>[2x]RPSGRKSSKMQAFRIWDVNQKTFYLRNNQLVAGYLQGPNVNLEEKIDVVPIEPHALFLGIHGGKMCLSCVKSGDETRLQLE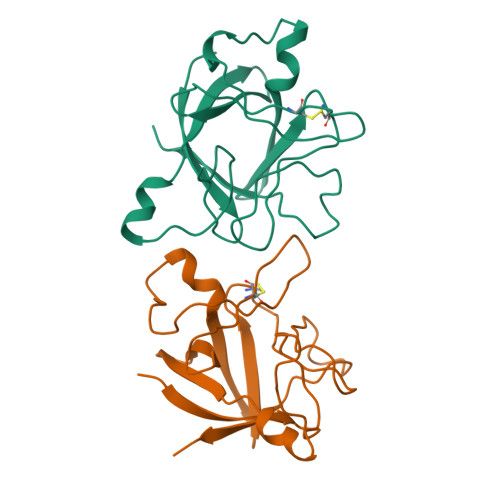AVNITDLSENRKQDKRFAFIRSDSGPTTSFESAACPGWFLCTAMEADQPVSLTNMPDEGVMVTKFYFQEDE>[2x]GEQAQQARELGQSLAQEVKAATERLSLGSRDVAERLRLSKDIGRLIEAVETSVMPQWQRRELLATVKMLQRRANTAIRKLQMGQAAKKTQELLERHSKGPLIVDTVSAESLSVLVKVVRQLCEQAPSTSVLLLSPQPMGKVLCACQVAQGAMPTFTAEAWALAVCSHMGGKAWGSRVVAQGTGSTTDLEAALSIAQTYALSQLL

Consistent with its absence from primate mt tRNAAla sequences, the human mt AlaRS/tRNAAla system was recently shown to be insensitive to a G3:U70 identity element. For the human mt AlaRS/tRNAAla system we show that loss of the G3:U70 identity element was accompanied by a radical reorganization of the recognition mechanism, away from sequence-specific direct readout in the acceptor stem to sequence-unspecific structural readout of the flexible tRNA elbow. The appended C-Ala domain, which plays an auxiliary role in prokaryotic AlaRSs and is dispensable for aminoacylation in the human cytoplasmic AlaRS system, plays a central role as a folding aid for the intrinsically flexible mt tRNA elbow. Fine-tuned induced-fit adaptation selects mt tRNAAla and rejects non-cognate mt tRNAs.

The model suggested two major contact sites between mt C-Ala and mt tRNAAla. One is in the C-terminal α/β-globular subdomain (aa 873 to C-terminus) containing the glycine-rich “GG” motif. The second is formed by helices α2 and α3 of the N-terminal subdomain (aa 783–872). Both helices are lined with highly conserved basic side chains that form an extended patch of positive surface charges. Due to the 3-helix architecture, helices α2 and α3 can move significantly closer to the tRNA than in the prokaryotic complex, allowing direct contacts with the T-stem and V-loop. In particular, the mt AlaRS-specific Gly825 appears to be important for tight association between C-Ala and tRNA and may explain the sensitivity to V-loop size (see above). Thus, adaptive evolution of the Hs mt AlaRS/tRNAAla recognition system was accompanied by a radical reorganization of its recognition system, moving the center for tRNA recognition from sequence-specific (G3:U70) readout in the acceptor stem to C-Ala-mediated sequence-unspecific readout of the tRNA’s elbow structure.>[6x]MAPKRKASSTCKTPKRQCIPKPGCCPNVASVPKLLVKGGVEVLSVVTGEDSITQIELYLNPRMGVNSPDLPTTSNWYTYTYDLQPKGSSPDQPIKENLPAYSVARVSLPMLNEDITCDTLQMWEAISVKTEVVGISSLINVHYWDMKRVHDYGAGIPVSGVNYHMFAIGGEPLDLQGLVLDYQTQYPKTTNGGPITIETVLGRKMTPKNQGLDPQAKAKLDKDGNYPIEVWCPDPSKNENSRYYGSIQTGSQTPTVLQFSNTLTTVLLDENGVGPLCKGDGLFISCADIVGFLFKTSGKMALHGLPRYFNVTLRKRWVKNPYPVVNLINSLFSNLMPKVSGQPMEGKDNQVEEVRIYEGSEQLPGDPDIVRFLDKFGQEKTVYPKPSVAPAAVTFQSNQQDKGKAPLKGPQKASQKESQTQEL

Merkel cell polyomavirus (MCPyV) is a human double-stranded DNA tumor virus. MCPyV cell entry is unique among members of the polyomavirus family as it requires the engagement of two types of glycans, sialylated oligosaccharides and sulfated glycosaminoglycans (GAGs). On the virus side, PyV-receptor interactions are mediated entirely by the major capsid protein VP1, which forms the capsid outer layer. VP1 assembles into 72 pentameric capsomers, giving rise to small capsids of 45 to 50 nm in diameter.

Using the fVLP preparation, we solved crystallographic and cryo-EM structures of the outer (VP1-only) MCPyV capsid. The structures have 3.5-Å and 3.4-Å resolutions, with no significant differences between them. In MCPyV, we observed clear density for five out of potentially six disulfide bridges that connect individual VP1 chains within the strict and local pentamers, respectively, i.e., for the α-α, α′-α″, α″-β, β-β′, and γ-α′ linkages. The crystallographic electron density shows unambiguously that only Cys25 is involved in the ringlike intracapsomer disulfide bridges, tethering each VP1 N terminus covalently to its clockwise (cw) neighbor’s CD-loop (residues 108 to 118) via Cys117, the mPyV Cys115 homolog. Additionally, the MCPyV crystal structure revealed unique intercapsomer disulfide bridges, rendered possible by the presence of two additional cysteines (Cys18 and Cys24). These two cysteines form two novel and distinct structural elements, which we term the trinity knot and disulfide handshake, respectively. The trinity knot is located at the interface between two local pentamers and one strict pentamer tethering each of the α-, α′-, and γ-chains to the respective other two. The disulfide handshake links two local pentamers whose chains run in an antiparallel fashion, with two simultaneous Cys18-Cys24 bridges (Cys18α″-Cys24β and Cys18β-Cys24α″). For our MCPyV capsids, we provided 1 mM calcium chloride in all buffers. The crystallographic electron density suggests the presence of only one divalent ion, coordinated by the Ser236 backbone carbonyl and Glu239 side chain carboxyl groups of one monomer as well as the Glu56 side chain of the neighboring monomer and the Glu353 side chain of an invading arm of another capsomer (counterclockwise [ccw]) [i.e., involving Ser236α′, Glu239α′, Glu56γ, and (ccw)Glu353γ].> ALTKAEMSEYLFDKLGLSKRDAKELVELFFEEIRRALENGEQVKLSGFGNFDLRDKNQRPGRNPKTGEDIPITARRVV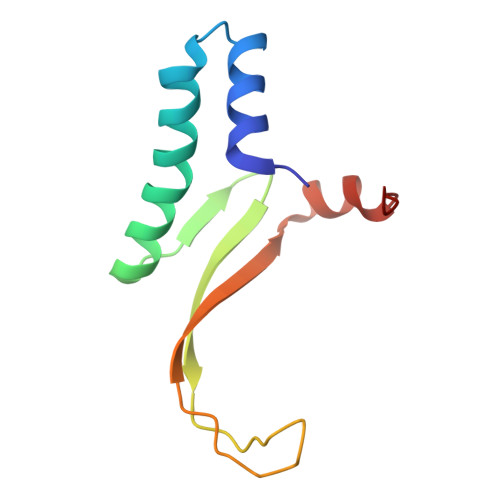TFRPGQKLKSRVENASPK>[3x]MSVSEIFVELQGFLAAEQDIREEIRKVVQSLEQTAREILTLLQGVHQGAGFQDIPKRCLKAREHFGTVKTHLTSLKTKFPAEQYYRFHEHWRFVLQRLVFLAAFVVYLETETLVTREAVTEILGIEPDREKGFHLDVEDYLSGVLILASELSRLSVNSVTAGDYSRPLHISTFINELDSGFRLLNLKNDSLRKRYDGLKYDVKKVEEVVYDLSIRGFNKETAAACVEK;> MSNKEGSGGFRKRKHDNFPHNQRREGKDVNSSSPVMLAFKSFQQELDARHDKYERLVKLSRDITVESKRTIFLLHRITSAPDMEDILTESEIKLDGVRQKIFQVAQELSGEDMHQFH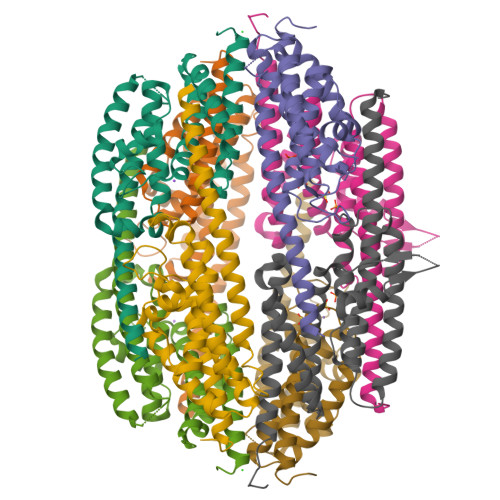RAITTGLQEYVEAVSFQHFIKTRSLISMDEINKQLIFTTEDNGKENKTPSSDAQDKQFGTWRLRVTPVDYLLGVADLTGELMRMCINSVGNGDIDTPFEVSQFLRQVYDGFSFIGNTGPYEVSKKLYTLKQSLAKVENACYALKVRGSEIPKHMLADVFSVKTEMIDQEEGIS>DEDQVDPRLIDGKWSRDQYHVLFDSYRDNIAGKSFQNRLCLPMPIDVVYTWVNGTDLELLKELQQVREQMEEEQKAMREILGKNTTEPTKKSEKQLECLLTHCIKVPMLVLDPALPANITLKDLPSLYPSFHSASDIFNVAKPKNPSTNVSVVVFDSTKDVEDAHSGLLKGNSRQTVWRGYLTTDKEVPGLVLMQDLAFLSGFPPTFKETNQLKTKLPENLSSKVKLLQLYSEASVALLKLNNPKDFQELNKQTKKNMTIDGKELTISPAYLLWDLSAISQSKQDEDISASRFEDNEELRYSLRSIERHAPWVRNIFIVTNGQIPSWLNLDNPRVTIVTHQDVFRNLSHLPTFSSPAIESHIHRIEGLSQKFIYLNDDVMFGKDVWPDDFYSHSKGQKVYLTWPVPNCAEGCPGSWIKDGYCDKACNNSACDWDGGDCSGNSGGSRYIAGGGGTGSIGVGQPWQFGGGINSVSYCNQGCANSWLADKFCDQACNVLSCGFDAGDCGQDHFHELYKVILLPNQTHYIIPKGECLPYFSFAEVAKRGVEGAYSDNPIIRHASIANKWKTIHLIMHSGMNATTIHFNLTFQNTNDEEFKMQITVEVDTREGPKLNSTAQKGYENLVSPITLLPEAEILFEDIPKEKRFPKFKRHDVNSTRRAQEEVKIPLVNISLLPKDAQLSLNTLDLQLEHGDITLKGYNLSKSALLRSFLMNSQHAKIKNQAIITDETNDSLVAPQEKQVHKSILPN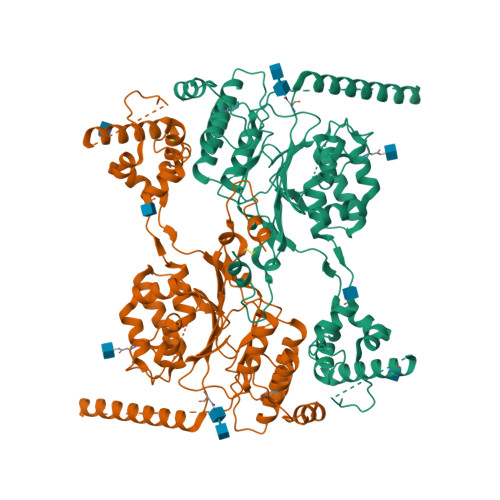SLGVSERLQRLTFPAVSVKVNGHDQGQNPPLDLETTARFRVETHTQKTIGGNVTKEKPPSLIVPLESQMTKEKKITGKEKENSRMEENAENHIGVTEVLLGRKLQHYTDSYLGFLPWEKKKYFQDLLDEEESLKTQLAYFTDSKNRARYKRDTFADSLRYVNKILNSKFGFTSRKVPAHMPHMIDRIVMQELQDMFPEEFDKTSFHKVRHSEDMQFAFSYFYYLMSAVQPLNISQVFDEVDTDQSGVLSDREIRTLATRIHELPLSLQDLTGLEHMLINCSKMLPADITQLNNIPPTQESYYDPNLPPVTKSLVTNCKPVTDKIHKAYKDKNKYRFEIMGEEEIAFKMIRTNVSHVVGQLDDIRKNPRKFVCLNDNIDHNHKDAQTVKAVLRDFYESMFPIPSQFELPREYRNRFLHMHELQEWRAYRDKLK[2x]>KNEPVLDIDGEELRAGEQYYVVSAIWGPGGGGLALGRLTDQKCPEIVVQRRSDSDYGTPVIFHNLDTKDDIVRLSTDFNVEFVPIRDRLCLTSTVWKIDDYDTSTGQWWVTTNGVIGNPGPQTLQSWFKIE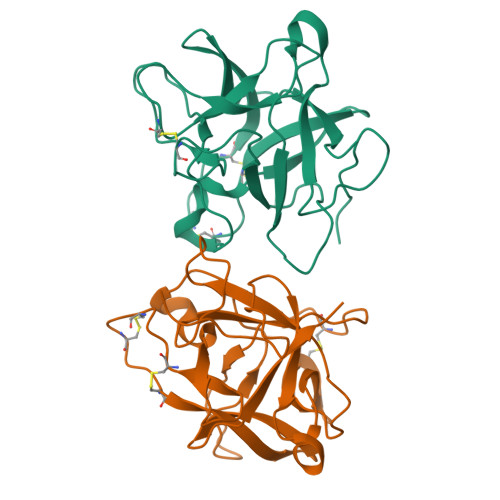KSGNLGYKFNFCPSVCESCVTLCSDIGRYGDDGQIRLALAERGWPFVFKKASSTIKQIVYAKN[2x]>MGSSHHHHHHSQDPMTQNADQYRVRKEPYYRAVQDEIELYRAGYEARIPMMLKGPTGCGKSRFVEHMAWKLNRPLITIACNEDMTASDLVGRYLLDKDGTRWQDGPLTVAARIGAICYLDEIVEARQDTIVVIHPLTDHRRVLPLEKKGELVEAHPDFQIVISYNPGYQSLMKDLKQSTKQRFGALDFDYPKPDIEAEIVSHEAGVDKDTAEKLVQIAQKARNLKGHGLDEGLSTRLLVYAGKLIAKGVDARAACTMTLVNPITDDVDMRDALDTVVK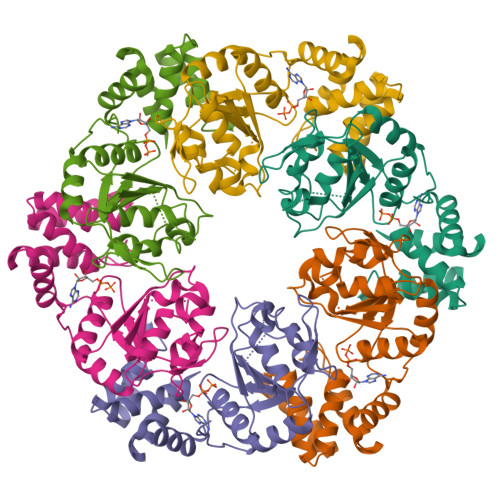TFF[2x]>MENTIRLIPFKIEE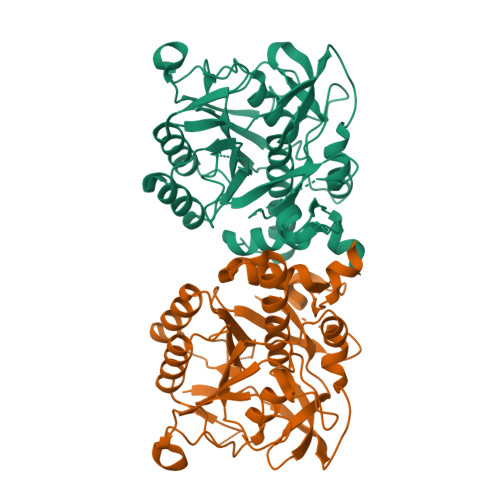KLESVKEIPEGVNMVQAPEIWKEGIRGKDIVIAVIDTGCDRDHPDLKDRIIGGRNFTTDDNGDVDNYSDYNGHGTHVAGTIAATENDQGVVGVAPEAKLLILKVLANDPNNPGSATGKYEWIVNAINYAIDQKVDIISMSLGGPSDVPELHQAVKRAVENNILVVCAAGNEGDGNERTEELSYPAAYNEVISVGAISLDGQISRFTNSNKEIDVVAPGEKILSTIPGGKFAVFSGTSMATPHVSGALALIKQLSEKEFERNLTEPELYAQLIKRTMPLGFPKALEGNGLVYLTAPNLLSRHYEKTQVSSILVPR[4x]> MANVNKTPGKTRRAEVAGGGFAGLTAAIALKQNGWDVRLHEKSSELRAFGAGIYLWHNGLRVLEGLGALDDVLQGSHTPPTYETWMHNKSVSKETFNGLPWRIMTRSHLHDALVNRARALGVDISVNSEAVAADPVGRLTLQTGEVLEADLIVGADGVGSK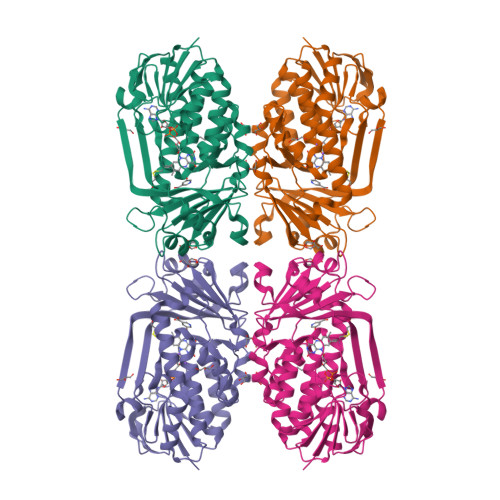VRDSIGFKQDRWVSKDGLIRLIVPRMKKELGHGEWDNTIDMWNFWPRVQRILYSPCNENELYLGLMAPAADPRGSSVPIDLEVWVEMFPFLEPCLIEAAKLKTARYDKYETTKLDSWTRGKVALVGDAAHAMCPALAQGAGCAMVNAFSLSQDLEEGSSVEDALVAWETRIRPITDRCQALSGDYAANRSLSKGNMFTPAALEAARYDPLRRVYSWPQ>[4x]PLKPEE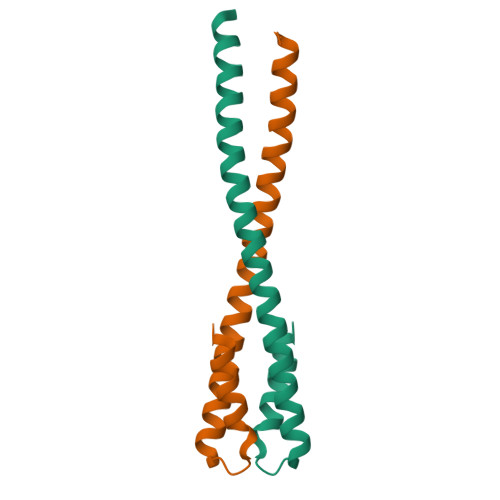HEDILNKLLDPELAQSERTEALQQLRVNYGSFVSEYNDLTKSHEKLAAEKDDLIVSNSKLFRQIGLTEKQEEDHKKADISETITIEDLEAK>MTAGSDRRPRDPAGRRQAIVEAAERVIARQGLGGLSHRRVAAEANVPVGSTTYYFNDLDALREAALAHAANASADLLAQWRS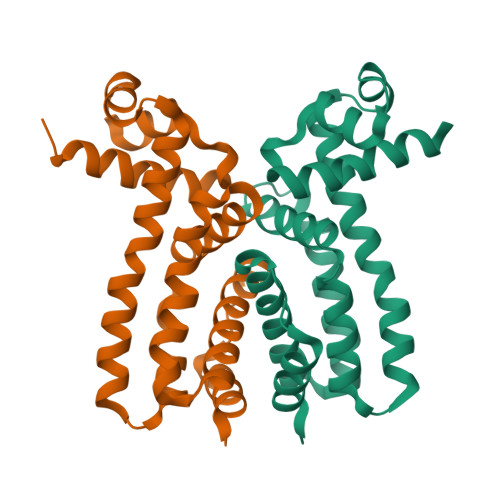DLDKDRDLAATLARLTTVYLADQDRYRTLNELYMAAAHRPELQRLARLWPDGLLALLEPRIGRRAANAVTVFFDGATLHALITGTPLSTDELTDAIARLVADGPEQREVGQSAHAGRTPDHHHHHH[2x]Here we describe the discovery and characterisation of endo-acting glycoside hydrolases expressed by mucin-degrading members of the HGM that are able to cleave the O-glycan chains of a range of different animal and human mucins. These O-glycanases display endo-β1,4-galactosidase activity and specifically target the polyLacNAc structures that comprise the main backbone of many mucin glycan chains. All of the GH16 enzymes comprise a β-jellyroll fold, characteristic of the family, consisting of two β-sheets composed of β-strands that form the core fold, which were superimposable with other GH16 structures previously published. Overall these data reveal that the nine GH16 enzymes analysed are endo acting β1,4-galactosidases that display a preference for polyLacNAc structures found in mucins and other similar glycans such as KS.

Structures of BF4060 and BACCAC_02680E143Q were also obtained with the Galβ1,4GlcNAcβ1,3 Gal product present in the negative subsites (despite the latter enzyme being a catalytic mutant) to 3.3 and 2.0 Å. A cleft running along the concave surface of the enzymes contains the active site and where the trisaccharide product was bound in the cases of BF4060 and BACCAC_02680E143Q. Inspection of the BACCAC_02680E143Q and BF4060 structures with product reveal most of the interactions between enzyme and sugar are with the Gal at −1 and GlcNAc at −2. BF4060 and BACCAC_02680E143Q have four fingers and BACCAC_03717 and Amuc_0724 have five out of six possible fingers that have been observed previously in other GH16 structures. BF4060 and BACCAC_02680 display 79% identity and unsurprisingly the structures of these two enzymes are almost identical in the cleft region. BF4060 (and also its close homologue BACCAC_02680) has a significant preference for TriLacNAc over milk oligosaccharides and analysis of the +1 subsite shows a narrow slot where a GlcNAc would insert with the N-acetyl pointing away from the cleft and S174 from Finger 5 would pincer the N-acetyl against finger 6, thus generating specificity for GlcNAc over glucose. BF4060, BACCAC_02680 and BACCAC_03717 also displayed some very weak activity against laminarin.

>SVLFVDSFDGSSVVPDTAVWKLCTYANNAWSQWFRDVNGYENVKVEDGYLKLRACKDNGTYKNGGVFSKIGFPCGTRLEVKARLTKLVRGGFPAIWQMPIGAPEWPRGGEIDLMEWVQGTPLQIYQTVHTYYINGANGSAGVTNKNPDKNFDVTKDHVYAVERTEKEVIFYVDGKETWRYGNQYLDEGKLQYPFCEYPFNIILNFSLGGELNGRMTWSGEICDEDLPGEMWVDWVRVVSLN[3x]> SRANDAPIVLLHGFTGWGREEMFGFKYWGGVRGDIEQWLNDNGYRTYTLAVGPLSSNWDRACEAYAQLVGGTVDYGAAHAAKHGHARFGRTYPGLLPELKRGGRIHIIAHSQGGQTARMLVSLLENGSQECREYAKAHNVSLSPLCEGGHHFVLSVTTIATPHDGTTLVNMVDFTDRFFDLQKAVLKAAAVASNVPYTS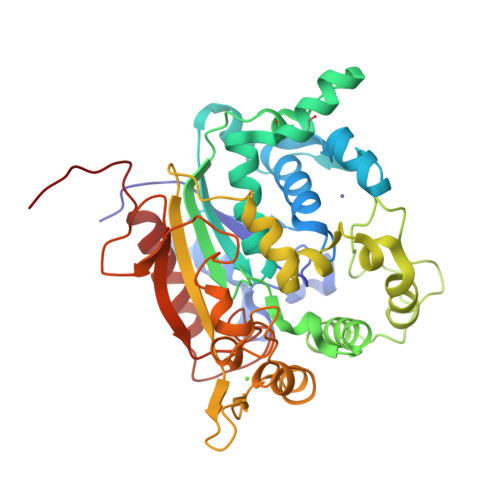QVYDFKLDQWGLRRQPGESFDQYFERLKRSPVWTSTDTARYDLSVPGAEKLNQWVKASPNTYYLSFATERTYRGALTGNYYPELGMNAFSAVVCAPFLGSYRNATLGIDDRWLENDGIVNAFSMNGPKRGSTDRIVPYDGTIKKGVWNDMGTYNVDHLEVIGVDPNPLFDIRAFYLRLAEQLASLQPHHHHHH Equine herpesvirus type 1 (EHV-1) and EHV-4 gDs interact with equine major histocompatibility complex I (MHC-I) to initiate entry into equine cells. Of these, gD is the (main) receptor-binding protein that interacts with the cell receptors and triggers the subsequent fusion process with cell membrane and/or uptake by endocytosis. The structures of gD1 and gD4 revealed the existence of a common V-set immunoglobulin-like (IgV-like) core comparable to those of other gD homologs. The cores consist of a nine-stranded (A′, B, C, C′, C″, D, E, F, and G) β-barrel, arranged in a typical V-like Ig fold, flanked by N- and C-terminal extensions with loops, α-helices (α1, α2, α3’, and α3), and small β-strands (str2-4).

Glycoprotein D4 was crystallized with one protein per asymmetric unit. In total 244 residues could be modeled (R34 to R277). The overall folds of gD1 and gD4 are very similar with a root-mean-square deviation (rmsd) of 0.7 Å for 220 common Cα atoms. In the structures of gD1 and gD4, six cysteines were found to form three disulfide bonds at sites conserved in members of the gD plolypeptide family: C87/C209, C126/C223, and C138/C147 (Carfi et al., 2001; Li et al., 2017; Yue et al., 2020). Apparent dissociation constants ( Kdapp ) of 7,000 ± 2,000 nM and 5,800 ± 760 nM were calculated for gD1 and gD4, respectively. Additionally, the receptor affinity of a C-terminally truncated EHV-4 gD, gD436-280, was tested. The truncated gD4 version, gD436-280, exhibited a receptor binding affinity to MHC-I in the same order of magnitude (6,700 ± 750 nM). That the C-terminal truncation had no significant effect on the receptor affinity of EHV-4 gD suggests that the mode of binding differs from other alphaherpesviruses, however, the role of the C-terminus remains to be determined. For EHV-4, the infection was reduced by an average of 32% after blocking the cells with soluble gD4 recombinant protein. gD4 was also able to block the entry of EHV-1 by 40%. The EHV-1 gD complex was one of the 3% best scored results and the EHV-4 gD complex was in the 11% top results suggesting that both docking solutions represent low-energy protein complexes.

> ENYRRVVRGNQNQRPEFPPPRYNFTIVTTYNETSLPSPFINDQVKIVDVRTVAATRPCEMIALIAKTNVDSIIKELDAAHKTYSARLTWFKITPTCATPIHDVVYMKCNPKLLFGMCDERSNILWLNSLITTAAETDDELGLVLASPAHSYSGLYRRVIQIDGRRIYTDFSVTIPSSHCPLSFEQNFGNPDRCKTPEQYSRGEVYTSRFLSEFNYRQGVHLAWVKHWFVQDGGNLPVQFYEAQAFARPVPPDNHPGFDSVESEITQNKTNPKQEQASPKPNPPFKWPSIKQLAPRIDEVDNAKEITTKKPPASNSNSTFENLYFQGHHHHHH> MKEQLEDVLDTLTDREENVL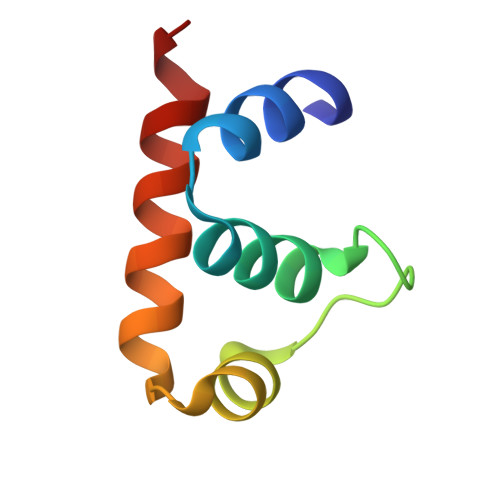RLRFGLDDGRTRTLEEVGKVFGVTRERIRQIEAKALRKLRHP> WSHPQFEKVPIKYLPEENVHDADFGEQKDISEINLAAGLDLFQGDILLQKSRNGLRDPNTRWTFPIPYILADNLGLNAKGAILYAFEMFRLKSCVDFKPYEGESSYIIFQQFDGCWSEVGDQHVGQNISIGQGCAYKAIIEHEILHALGFYHEQSRTDRDDYVNIWWDQILSGYQHNFDTYDDSLITDLNTPYDYESLMHYQPFSFNKNASVPTITAKIPEFNSIIGQRLDFSAIDLERLNRMYNCTTTHTLLDHCTFEKANICGMIQGTRDDTDWAHQDSAQAGEVDHTLLGQCTGAGYFMQFSTSSGSAEEAALLESRILYPKRKQQCLQFFYKMTGSPSDRLVVWVRRDDSTGNVRKLVKVQTFQGDDDHNWKIAHVVLKEEQKFRYLFQGTKGDPQNSTGGIYLDDITLTETPCPTGVWTVRNFSQVLENTSKGDKLQSPRFYNSEGYGFGVTLYPNSRESSGYLRLAFHVCSGENDAILEWPVENRQVII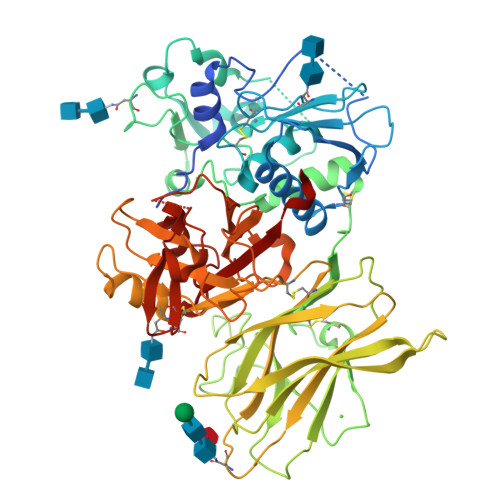TILDQEPDVRNRMSSSMVFTTSKSHTSPAINDTVIWDRPSRVGTYHTDCNCFRSIDLGWSGFISHQMLKRRSFLKNDDLIIFVDFEDITHLS>CGC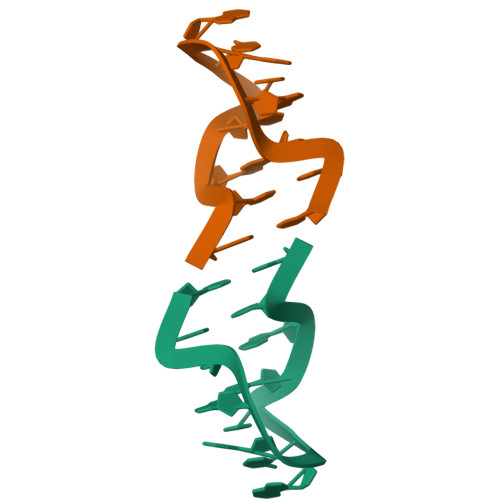GAAXXCGCG[2x]> GAMA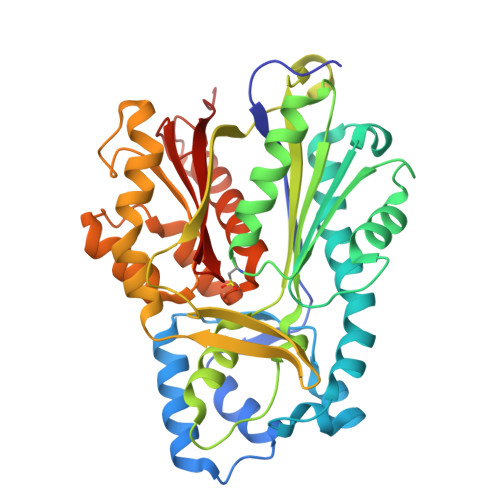NHLRAEGPASVLAIGTANPENILLQDEFPDYYFRVTKSEHMTQLKEKFRKICDKSMIRKRNCFLNEEHLKQNPRLVEHEMQTLDARQDMLVVEVPKLGKDACAKAIKEWGQPKSKITHLIFTSASTTDMPGADYHCAKLLGLSPSVKRVMMYQLGCYGGGTVLRIAKDIAENNKGARVLAVCCDIMACLFRGPSESDLELLVGQAIFGDGAAAVIVGAEPDESVGERPIFELVSTGQTILPNSEGTIGGHIREAGLIFDLHKDVPMLISNNIEKCLIEAFTPIGISDWNSIFWITHPGGKAILDKVEEKLHLKSDKFVDSRHVLSEHGNMSSSTVLFVMDELRKRSLEEGKSTTGDGFEWGVLFGFGPGLTVERVVVRSVPIKY>[2x]GMTSGAGWEEQVFLPITNS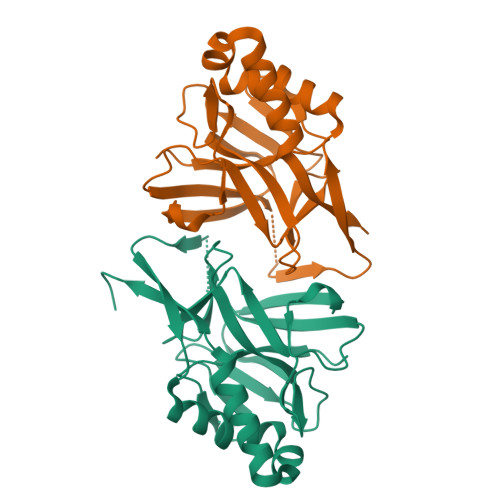ISSEDNNQIKIGSSVSIEYNQNGQHVSQIDDKGLHNILVLTGYAIDESTGELVPTFDPCDYVKGILISGKILKGNHFKIIGIPSNKLYIIRKKDVHGNITFSLPIKNFNTGTYQVDLRDKVTSFVSLDRDVAKTIVDNVLAKIYAKIYNSLNKEQKDKLYRDVEEIFNYYSIKSLKSNP>MEYDAFITNQLRGAQNQSSGLTTRYEQMSKIDNLLADKSSSLSGSLQSFFTSLQTLVSNAEDPAARQALIGKAEGLVNQFKTTDQYLRDQDKQVNIAIGSSVAQINNYAKQIANLNDQISRMTGVGAGASPNDLLDQRDQLVSELNKIVGVEVSVQDGGTYNLTMANGYTLVQGSTARQLAAVPSSADPTRTTVAYVDEAAGNIEIPEKLLNTGSLGGLLTFRSQDLDQTRNTLGQLALAFADAFNAQHTKGYDADGNKGKDFFSIGSPVVYSNSNNADKTVSLTAKVVDSTKVQATDYKIVFDGTDWQVTRTADNTTFTATKDADGKLEIDGLKVTVGTGA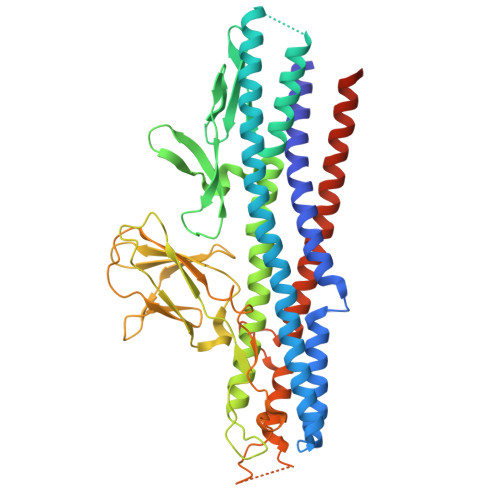QKNDSFLLKPVSNAIVDMNVKVTNEAEIAMASESKLDPDVDTGDSDNRNGQALLDLQNSNVVGGNKTFNDAYATLVSDVGNKTSTLKTSSTTQANVVKQLYKQQQSVSGVNLDEEYGNLQR[2x]>[2x]GTIYPRNPAMYSEEARLKSFQNWPDYAHLTPRELASAGLYYTGIGDQVQCFACGGKL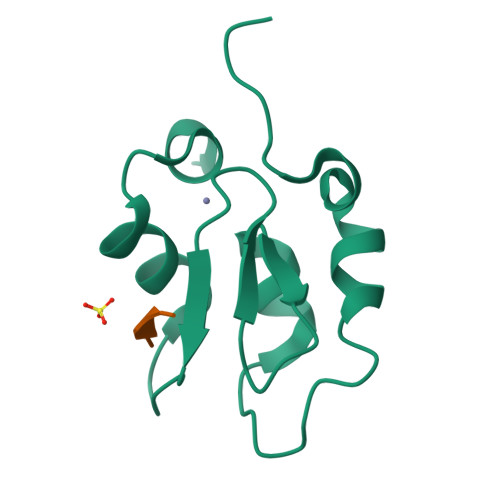KNWEPGDRAWSEHRRHFPNCFFVLGRNLN;> AMRV> MGSSHHHHSQASMITRYKPESGFVARSGGPDRKRPHDWIVWHFTHADNLPGIITAGRLLADSAVTPTTEVAYNPVKELRRHKVVAPDSRYPASMASDHVPFYIAARSPMLYVVCKGHSGYSGGAGPLVHLGVALGDIIDADLT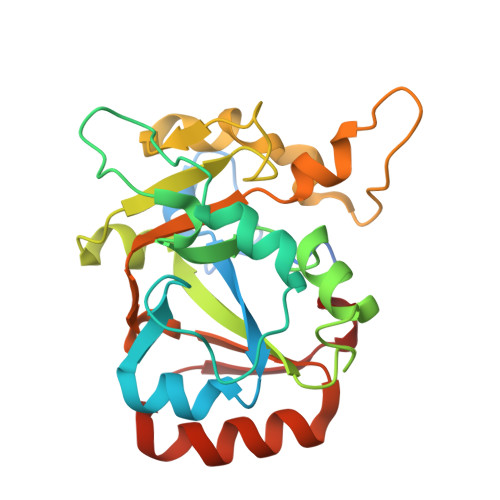WCASDGNAAASYTKFSRQVDTLGTFVDFDLLCQRQWHNTDDDPNRQSRRAAAILVYGHVPFELVSYVCCYNTETMTRVRTLLDPVGGVRKYVIKPGMYY> MAKLPYSRVTNVTLTRTDNFPTRRGFGTQLILTHTAVSGQVDATKRTKLYASLAEVEADYPANTSVYKAALSAFSQNPRPIRLKVGYAATPTGGDDAAKKADFITSLGAILNYDQAFYQITLDAALRDQPYLDGLVEWVEAQPKIAMIDSNAAGHEDPANTTVIAARHKGTVERTAVFYHTDSTEYLAA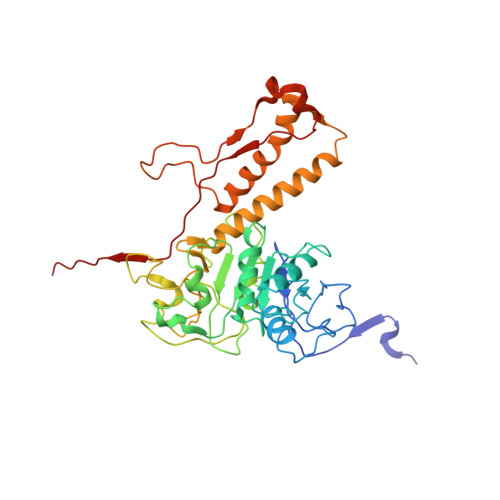SMAAYMSTRVFDDANSAYTLKFKKAPGVRAIDKGSAVVTAITGFVEQTGQSESAGHCANTLIDIGDQEFLVEGSTLTQNVFLDEIHATDWIIARTEEEMLSLFLNNDRVPFTDQGMQQLASVPRAIMQLAARAGIVALDLNPLTGAYEPAYTITVPSVFDIPESQRKARIAPAIQVRFRYAGAVHYSVINYTMTF> SESQLKKMVSKYKYRDLTVRETVNVITLYKDLKPVLDSYVFNDGSSR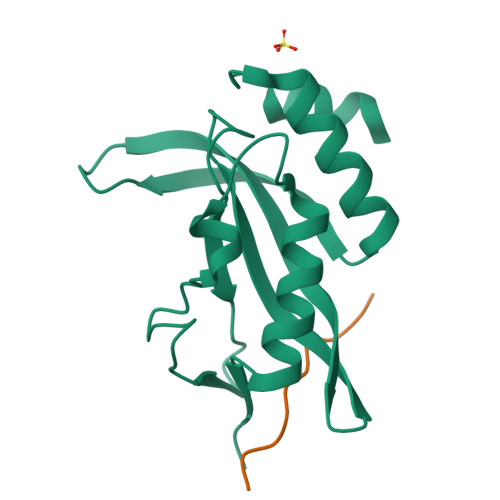ELMNLTGTIPVPYRGNTYNIPICLWLLDTYPYNPPICFVKPTSSMTIKTGKHVDANGKIYLPYLHEWKHPQSDLLGLIQVMIVVFGDEPPVFSRP;> YVEPTAPQVL>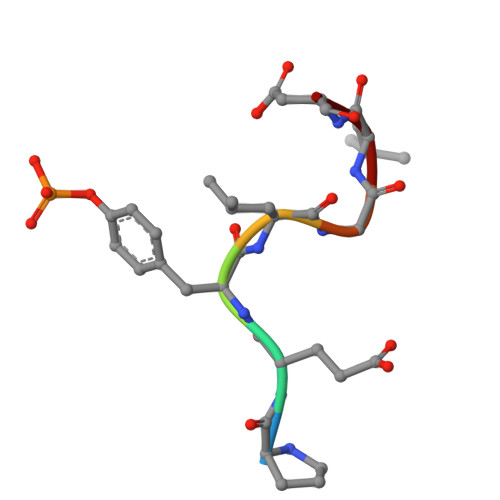 PEYLGLD>[3x]AEYCFNMNFIKDNSRALIQRMGMTVIKQITDDLFVWNVLNREEVNIICCEKVEQDAARGIIHMILKKGSESCNLFLKSLKEWNYPLFQDLNGQSLFHQTSEGDLDDLAQDLKDLYHTPSFLNFYPLGEDIDIIFNLKS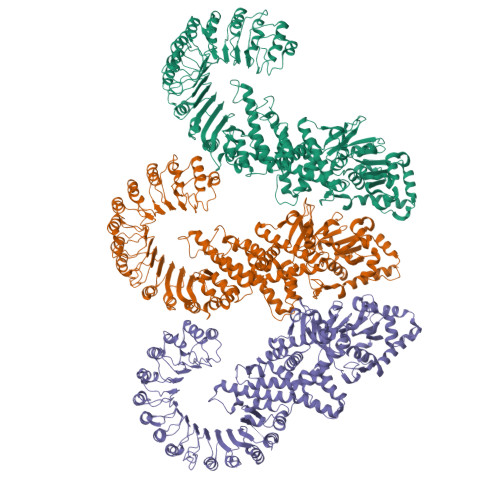TFTEPVLWRKDQHHHRVEQLTLNGLLQALQSPCIIEGESGKGKSTLLQRIAMLWGSGKCKALTKFKFVFFLRLSRAQGGLFETLCDQLLDIPGTIRKQTFMAMLLKLRQRVLFLLDGYNEFKPQNCPEIEALIKENHRFKNMVIVTTTTECLRHIRQFGALTAEVGDMTEDSAQALIREVLIKELAEGLLLQIQKSRCLRNLMKTPLFVVITCAIQMGESEFHSHTQTTLFHTFYDLLIQKNKHKHKGVAASDFIRSLDHCGDLALEGVFSHKFDFELQDVSSVNEDVLLTTGLLCKYTAQRFKPKYKFFHKSFQEYTAGRRLSSLLTSHEPEEVTKGNGYLQKMVSISDITSTYSSLLRYTCGSSVEATRAVMKHLAAVYQHGCLLGLSIAKRPLWRQESLQSVKNTTEQEILKAININSFVECGIHLYQESTSKSALSQEFEAFFQGKSLYINSGNIPDYLFDFFEHLPNCASALDFIKLDFYGGAMASWEKAAEDTGGIHMEEAPETYIPSRAVSLFFNWKQEFRTLEVTLRDFSKLNKQDIRYLGKIFSSATSLRLQIKRCAGVAGSLSLVLSTCKNIYSLMVEASPLTIEDERHITSVTNLKTLSIHDLQNQRLPGGLTDSLGNLKNLTKLIMDNIKMNEEDAIKLAEGLKNLKKMCLFHLTHLSDIGEGMDYIVKSLSSEPCDLEEIQLVSCCLSANAVKILAQNLHNLVKLSILDLSENYLEKDGNEALHELIDRMNVLEQLTALMLPWGCDVQGSLSSLLKHLEEVPQLVKLGLKNWRLTDTEIRILGAFFGKNPLKNFQQLNLAGNRVSSDGWLAFMGVFENLKQLVFFDFSTKEFLPDPALVRKLSQVLSKLTFLQEARLVGWQFDDDDLSVITGAFKLVTA>[2x]MRGSHHHHHHGSMKPYVLKFQEIRPHSEALVGGKGMNLGACSNIEGVHVPAGFCLTTEAYKRTLAENNEFTQLLQRLSSLKTSDMDAIREISETIRTLIQHTQIPSEIASYMDATLLDVGGYEMPFAVRSSATAEDLPHASFAGQHDTYLNIIGKDAL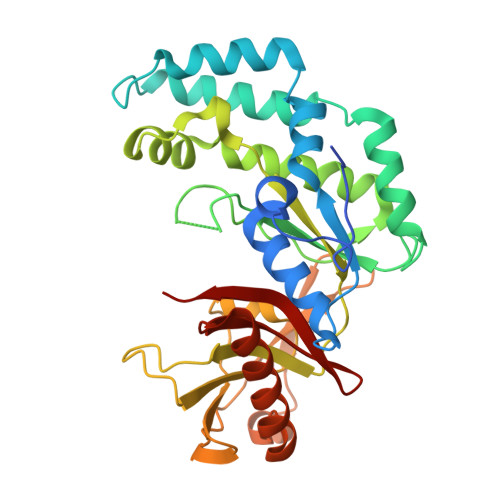LQHISMCWASLFTERAIIYRIQNQFDHRKVQLAVVIQQMISPEASGILFTADPITSNRKSLSIDASFGLGEALVSGLVSADSYTVRENTITNKIIATKKLAIYSLKEGGTETRILEKSQQTKQTLTDQQIIQLAKLGRKIEAYFGKPQDIEWCLAEGAFYIVQSRPITT> MKILKTLTLRGPNYWSIRRKKLIVMRLDLEDLAERPSNSIPGFYEGLIKVLPSLVEHFCSPGYQGGFLERVKEGTYMGHIVQHVALELQELVGMTAGFGRTRETSTPGVYNVVYEYVDEQAGRYAGRAAVRLCRSLVDTGDYPRLELEKDLEDLRDLGANSALGPSTETIVTEAEARKIPWMLLSARAMVQLGYGVYQQRIQATLSSHSGILGVELACDKEGTKTILQDAGIPVPRGTTIQYFDDLEEAINDVGG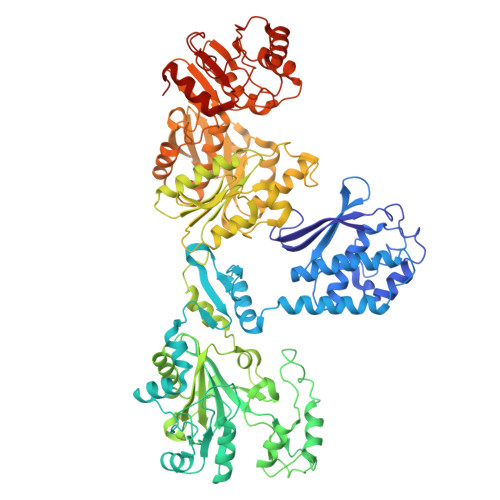YPVVIKPLDGNHGRGITINVRHWQEAIAAYDLAAEESKSRAIIVERYYEGSDHRVLVVNGKLVAVAERIPAHVTGDGSSTISELIEKTNQDPNRGDGHDNILTKIVVNKTAIDVMERQGYNLDSVLPKDEVVYLRATANLSTGGIAIDRTDDIHPENIWLMERVAKVIGLDIAGIDVVTSDISKPLRETNGVIVEVNAAPGFRMHVAPSQGLPRNVAAPVLDMLFPPGTPSRIPILAVTGTNGKTTTTRLLAHIYRQTGKTVGYTSTDAIYINEYCVEKGDNTGPQSAGVILRDPTVEVAVLETARGGILRAGLAFDSCDVGVVLNVAADHLGLGDIDTIEQMAKVKSVIAEVVDPSGYAVLNADDPLVAAMADKVKAKVAYFSMNPDNPIIQAHVRRNGIAAVYESGYLSILEGSWTLRVEQAKLIPMTMGGMAPFMIANALAACLAAFVNGLDVEVIRQGVRTFTTSAEQTPGRMNLFNLGQHHALVDYAHNPAGYRAVGDFVKNWQGQRFGVVGGPGDRRDSDLIELGQIAAQVFDRIIVKEDDDKRGRSEGETADLIVKGILQENPGASYEVILDETIALNKALDQVEEKGLVVVFPESVTRAIDLIKVRNPIGENLYFQ3-(3,4-dihydroxyphenyl)-7-hydroxy-4H-chromen-4-one | 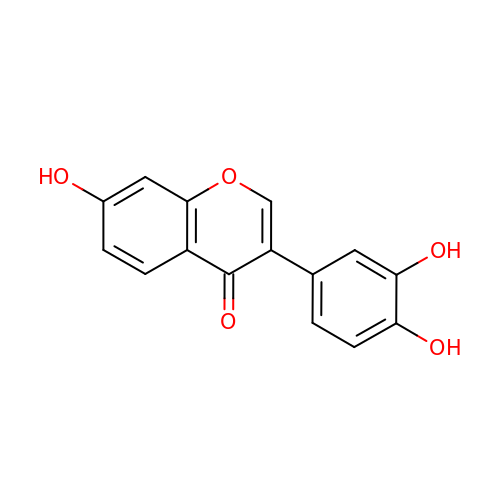C15 H10 O5 | DDKGKOOLFLYZDL-UHFFFAOYSA-N> EEYSSNWAGAVLIGDGYTKVTGEFTV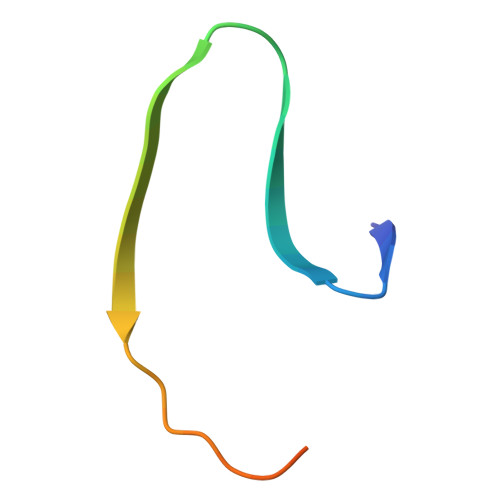PSVSAGSSGSSGY> MEANGLGPQGFPELKNDTFLRAAWGEETDYTPVWCMRQAGRYLPEFRETRAAQDFFSTCRSPEACCELTLQPLRRFPLDAAIIFSGILVVPQALGMEVTMVPGKGPSFPEPLREEQDLERLRDPEVVASELGYVFQAITLTRQRLAGRVPLIGFAGAPWTLMTYMVEGGGSSTMAQAKRWLYQRPQASHQLLRILTDALVPYLVGQVVAGAQALQLFESHAGHLGPQLFNKFALPYIRDVAKQVKARLREAGLAPVPMIIFAKDGHFALEELAQAGYEVVGLDWTVAPKKARECVGKT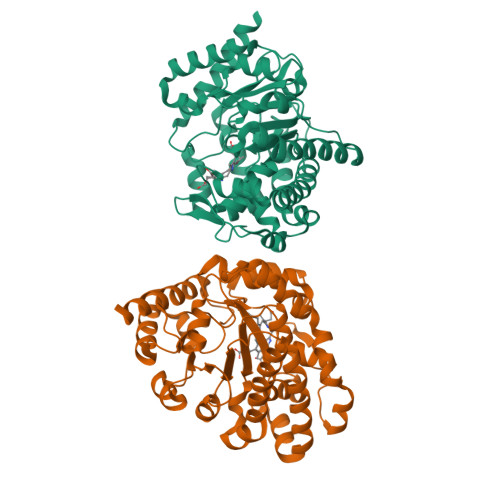VTLQGNLDPCALYASEEEIGQLVKQMLDDFGPHRYIANLGHGLYPDMDPEHVGAFVDAVHKHSRLLRQN(1R,2R)-2-(3-fluorobenzyl)-N-{2-[2-(1H-imidazol-1-yl)pyrimidin-4-yl]ethyl}cyclopropanamine | C19 H20 F N5 | 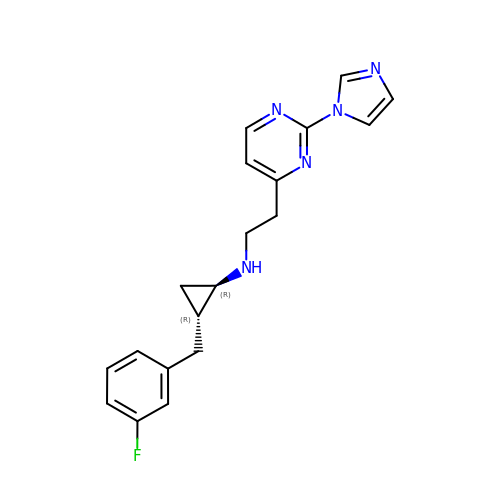CYEVFFVOLRMDHH-CRAIPNDOSA-N> MIALVLGLTSLACKPSGTVDPSIAQADQAGQADPLALYDLLEGRIAAGTDSEADRVAALEQVRAAADDQSAAYAYVRAAVAGRVAEGRGLKALKLLEEMRTWALTSIERDPGYRD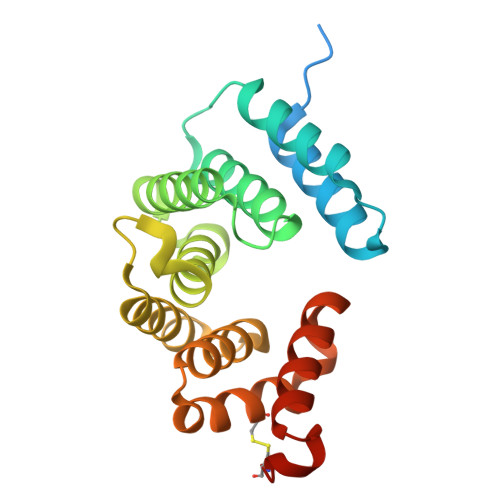MAATRMLGTLYVLAGQHLADGDSEQGLELLEDVVAAHPEAPTNHLRLAEGYIALGDPEPAFPSLCLAQGARAQLSGEEQRLLDGLLADIGGADLLACDAGGGS Mitogen-activated protein kinase kinase kinase kinase 1 (MAP4K1) is a serine/threonine kinase that acts as an immune checkpoint downstream of T-cell receptor stimulation. MAP4K1 activity is enhanced by prostaglandin E2 (PGE2) and transforming growth factor beta (TGFβ), immune modulators commonly present in the tumor microenvironment. Therefore, its pharmacological inhibition is an attractive immuno-oncology concept for inducing therapeutic T-cell responses in cancer patients. Through its proline-rich domain, MAP4K1 binds to a diversity of adaptors in hematopoietic cells, including those involved in T-cell receptor (TCR), B-cell receptor, and cytokine-induced signaling. The function of MAP4K1 has been studied most extensively in the context of T-cell activation.

We found that replacement of the pyrimidine with ureas such as 2 increased potency 10-fold, delivering single digit nanomolar inhibitors (IC50 = 7 nM). Protein X-ray crystallography confirmed that the urea moiety interacts in a bidentate hydrogen bond with the Asp101 side chain in MAP4K1 (Asp112 in the surrogate kinase MST1). Despite this increase in potency, selectivity toward ROCK2 remained a challenge. Ureas synthesized from cyclic amines, which reduced overall H-bond donors by one (not shown), also displayed more than a 10-fold decrease in activity, highlighting the importance of the two hydrogen bonds for overall potency.

>DIFNRDPRDHYDLLQRLGGGTYGEVFKARDKVSGDLVALKMVKMEPDDDVSTLQKEILILKTCRHANIVAYHGSYLWLQKLWICMEFCGAGSLQDIYQVTGSLSELQISYVCREVLQGLAYLHSQKKIHRDIKGANILINDAGEVRLADFGISAQIGATLARRLSFIGTPYWMAPEVAAVALKGGYNELCDIWSLGITAIELAELQPPLFDVHPLRVLFLMTKSGYQPPRLKEKGKWSAAFHNFIKVTLTKSPKKRPSATKMLSHQLVSQPGLNRGLILDLLDKLKNPG[2x]> MRIERVDDTTVKLFITYSDIEARGFSREDLWTNRKRGEEFFWSMMDEINEEE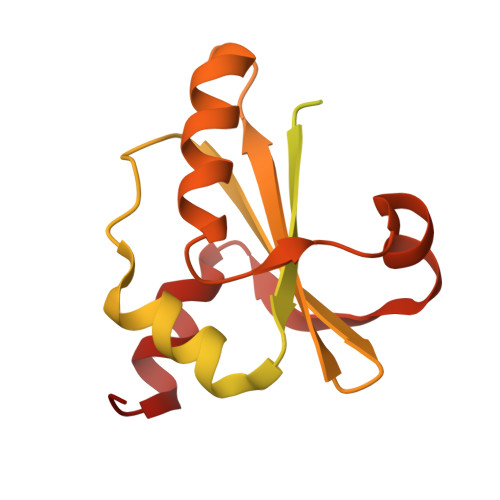DFVVEGPLWIQVHAFEKGVEVTISKSKNEDMMNMSDDDATDQFDEQVQELLAQTLEGEDQLEELFEQRTKEKEAQGSKRQKSSARKNTRTIIVKFNDLEDVINYAYHSNPITTEFEDLLYMVDGTYYYAVYFDSHVDQEVINDSYSQLLEFAYPTDRTEVYLNDYAKIIMSHNVTAQVRRYFPETTE> MKTITLYLDPASLPALNQLMDFTQNNEDKTHPRIFGLSRFKIPDNIITQYQNIHFVELKDNRPTEALFTILDQYPGNIELNIHLNIAHSVQLIRPILAYRFKHLDRVSIQQLNLY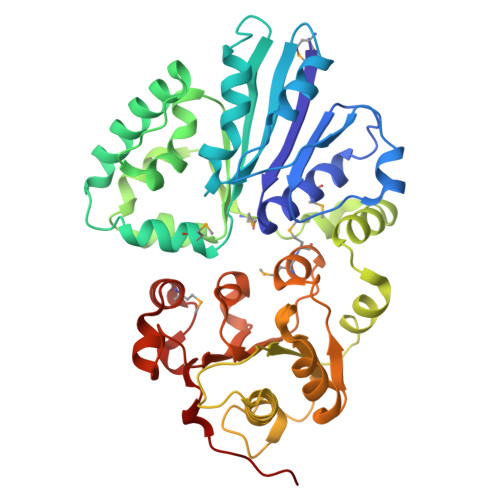DDGSMEYVDLEKEENKDISAEIKQAEKQLSHYLLTGKIKFDNPTIARYVWQSAFPVKYHFLSTDYFEKAEFLQPLKEYLAENYQKMDWTAYQQLTPEQQAFYLTLVGFNDEVKQSLEVQQAKFIFTGTTTWEGNTEVREYYAQQQLNLLNHFTQAEGDLFIGDHYKIYFKGHPRGGEINDIILNNAKNITNIPANISFEVLMMTGLLPDKVGGVASSLYFSLPKEKISHIIFTSNKQVKSKEDALNNPYVKVMRRLGIIDESQVIFWDSLKELGGG> ADDKSGKAPVITVFDHRGCQRGGPDREYKGKKANGPDDEMCVKVQSAKIAVSATT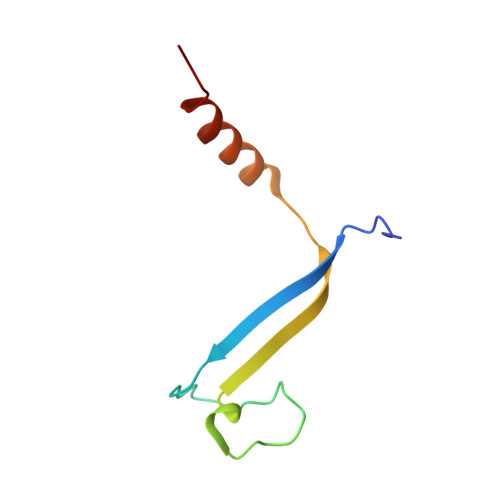ADSVLQQTISTLYRK>[2x]STHFDVIVVGAGSMGMAAGYQLAKQGVKTLLVDAFDPPHTNGSHHGDTRIIRHAYGEGREYVPLALRSQELWYELEKETHHKIFTKTGVLVFGPKGESAFVAETMEAAKEHSLTVDLLEGD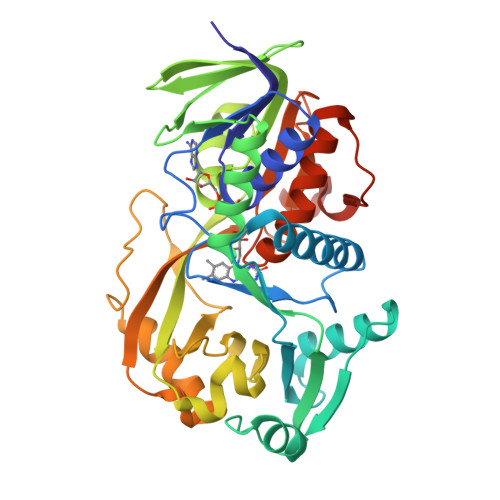EINKRWPGITVPENYNAIFEPNSGVLFSENCIRAYRELAEARGAKVLTHTRVEDFDISPDSVKIETANGSYTADKLIVSMGAWNSKLLSKLNLDIPLQPYRQVVGFFESDESKYSNDIDFPGFMVEVPNGIYYGFPSFGGCGLRLGYHTFGQKIDPDTINREFGVYPEDESNLRAFLEEYMPGANGELKRGAVCMYTKTLDEHFIIDLHPEHSNVVIAAGFSGHGFKFSSGVGEVLSQLALTGKTEHDISIFSINRPALKESLQKTTI Although it is annotated DsbA-like, PmScsC is a powerful protein disulfide isomerase that is able to refold and reactivate the scrambled disulfide form of the model substrate RNase A just as rapidly as the archetypal disulfide isomerase E. coli DsbC. Unexpectedly, evidence from chemical cross-linking, small angle X-ray solution scattering and multi-angle light scattering all indicated that PmScsC is trimeric. The N-terminal residues bring three catalytic domains together into a trimer, and a unique flexible linker enables extraordinary twisting and extending motions that impact on the catalytic domain placement. The combination, extent and diversity of these motions would enable mis-folded substrates bound to PmScsC to explore a broad folding landscape, consistent with the redox foldase activity of this key P. mirabilis copper resistance protein.

The three crystal structures—which we refer to as compact, transitional and extended —reveal an extraordinary range of motion in this protein. Importantly, the compact and transitional structures have multiple protomers in the asymmetric unit that adopt the same overall structures in each case (8 compact trimers, RMSD ∼1.5 Å for 645 Cα; two transitional trimers, RMSD 0.5 Å for 653 Cα) so that crystal symmetry does not appear to impact on the observed conformation. Moreover, the compact and transitional conformations were determined from crystals grown under similar conditions (2.85 M sodium malonate pH 5.8, 20 °C with either 0.1 M cobalt or copper added). Nevertheless, comparison of the eight compact and the two transitional trimers in these two crystal structures, reveals an unprecedented level of conformational re-arrangement (RMSDs>20 Å). In the 24 protomers present in the compact PmScsC crystal structure, the linker forms a loop that positions the three catalytic domains close to the trimerization stalk. The eight compact PmScsC trimers are mushroom-shaped with dimensions 80 × 80 × 50 Å3. The two compact protomer conformations of the transitional structure are similar to those in the compact crystal structure (RMSD 0.9–1.8 Å for 188 Cα).

>[24x]SNAALNAAQEKEVRALVRDTLVSNPEILEEAIMALQTKKADEQQAQFRQALASEHDALYNDAASPRIGAKDAKLVLVSFTDYNCPYCKRFDPLLEKITEQYPDVAVIIKPLPFKGESSAKASQAVLSVWKEDPKAFLALHQRLMQKKTMLDNASIEDAMKSTNTSKIKLTDDSLKTLQNNLELSRKLGIQGTPATVIGDTILPGAVDYDQLEIIVKEQLAKVKK Recently, RNA-catalyzed rolling circle synthesis (RCS) on small circular RNA (scRNA) templates has been demonstrated. To gain deeper insight into the RCS process and the strong inhibition observed upon full-length circle synthesis, we used cryo-EM to study the structure of putative RCS replication products formed by complexing the full-length scRNA and nascent complementary RNA (cmpRNA). To our surprise, cryo-EM revealed not one by a diverse variety of distinct structural species identified as monomers, dimers, and multimers of the scRNA–cmpRNA complex. We find that scRNAs and cmpRNAs of 36 nt in length can form an unanticipated diversity of structures with different stoichiometries, including a fully annealed dimer (comprising two scRNAs and two cmpRNAs) and multimers hereof.

Classes 4 and 5 represent multimers formed by end-to-end stacking of the class 3 dimers. The density maps for classes 4 and 5 could be readily modeled by stacking class 3 dimers to form twisted filaments—with class 4 comprising two dimers and class 5 three dimers. These multimer models suggest that the interaction between dimer units in the filament is mediated by base stacking of terminal bases from each unit. Based on the models, we suggest that A20 and G21 of one circular strand stacked with G21 and A20 of the other circular strand, respectively, and the 5′-end U1 of one unit stack on the U1 of the second unit, while the 3′-ends were nonstacking. The described distortion in the complex caused a global twist in the filament (period of ∼4 dimer units/turn). Notably, the 22–14 segmentation of the dimer also leads to a misalignment of the 5′- and 3′-ends of adjacent units. We observed a more intense low-mobility ligation band for the 33-nt circle compared to the 36-nt circle, supporting our observed misalignment of the 5′- and 3′-ends in class 4 and 5 models. In step 2, class 3 dimers assemble into multimers by end-to-end stacking, leading to the filament-like class 4 and 5 structures. The stable structure of the dimer furthermore allows multimers to form by end-to-end stacking.

>[4x]UGGAAGAAAUCGAAGAAGAUGAAGAACGCGAAGAAC;>[4x]AUCUUCUUCGAUUUCUUCCAGUUCUUCGCGUUCUUC> GSHMNIITVTLNMEKYNFLGISIVGQSNERGDGGIYIGSIMKGGAVAADGRIEPGDMLLQVNDMNFENMSNDDAVRVLRDIVHKPGPIVLT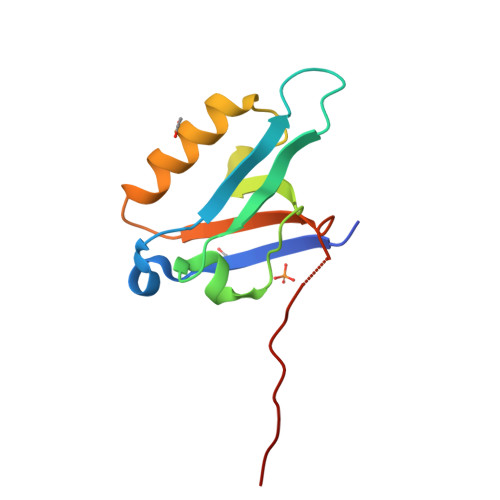VAKSGGGSGNEVWIDGP4-chloranyl-1-[(4-methoxy-3,5-dimethyl-pyridin-2-yl)methyl]pyrazolo[3,4-d]pyrimidin-6-amine 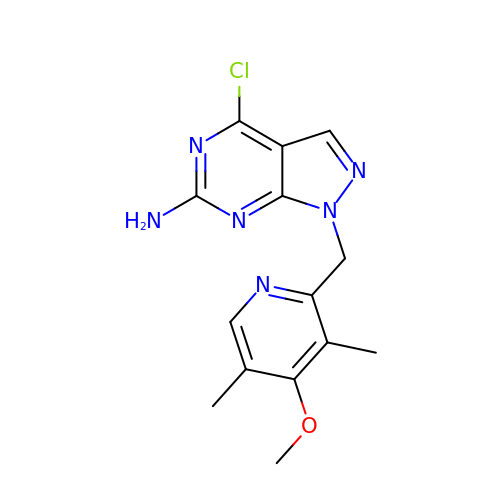| C14 H15 Cl N6 O | IKGRZHVFOMUXCQ-UHFFFAOYSA-N Coproheme decarboxylases (ChdCs) are enzymes produced by Gram‐positive bacteria that are involved in the coproporphyrin‐dependent pathway (CPD) of heme biosynthesis (Dailey et al. 2010; Dailey et al. 2017; Layer 2021; Pfanzagl et al. 2018; Zamarreño Beas et al. 2022). All ChdCs are homopentameric proteins consisting of protomers of 250–300 amino acid residues, each with two ferredoxin‐like domains, with only the C‐terminal domain having a functional coproheme/heme b binding site (Falb et al. 2023). The enzyme catalyzes the final two‐step decarboxylation of two propionate groups in the substrate iron coproporphyrin III (coproheme) to convert it into the final product heme b (Celis et al. 2017; Dailey et al. 2015; Lobo et al. 2015). In this study, we used cryogenic electron microscopy single‐particle reconstruction (cryo‐EM SPR) to characterize structurally the apo and heme b‐bound forms of actinobacterial coproheme decarboxylase from Corynebacterium diphtheriae.

The apo‐CdChdC cryo‐EM structure adds significantly to the structural knowledge on coproheme decarboxylases, it is also the first reported actinobacterial apo‐ChdC structure. It shows a complete absence of loop (108–127) densities for all five subunits. Missing densities can also be observed for the N‐terminal regions. In the cryo‐EM structure of heme b‐CdChdC, amino acid residues N6‐G235 were observed, while in apo‐CdChdC N11–P111 and S117–G235 residues were observed but there was no density for the N‐terminal residues as well as A112–R116 due to disorder. In principle, multiple distinct conformers of the loop can be resolved in cryo‐EM structures but dynamic disorder that we expect here averages out molecular density. As a result, in the 3D reconstructed map of the apo structure the loop density is only partially visible (Wu and Lander, 2020). The conformational change of the loop (L108–I127) in the apo structure seems to be accompanied by some additional conformational disorder of the N‐terminal residues (M1–L10) as they are located close to each other. The apo form of the protein exhibits greater conformational variability, as indicated by the lower accumulated populations of the first five clusters (78.5% for apo vs. 92.7% of the heme b complex). The apo form shows increased RMSF of loops 108–127 in both clusters 0 and 1 compared to the heme b complex; however, the effect is more significant for cluster 1 (open loop). This implies that the loop has increased flexibility in the absence of heme b, which is consistent with our cryo‐EM data indicating a lack of loop density in the apo structure.

>[5x]GPMAEKLNFEELNSMQRYSQFAVFRAIPGALGSDRAEIVAQAQSFFDGLETAGKVEVRGIYDLAGCRAEADFMIWWIAEEFEEIQAAFARFRRETVLGQVSEVAWLGNSLHRPAEFNRSHLPSFIMGEIPGDWITVYPFVRSYDWYIMDPQKRRKILAEHGQAARDFPDVRANTVPAFALGDYEWMLAFEAPRLDRIVDLMHKMRYTEARLHVREETPFFTGRRVSEVSELVNVLPG> GSRPSTAKPSKIPTPQRKSPASKLDKSS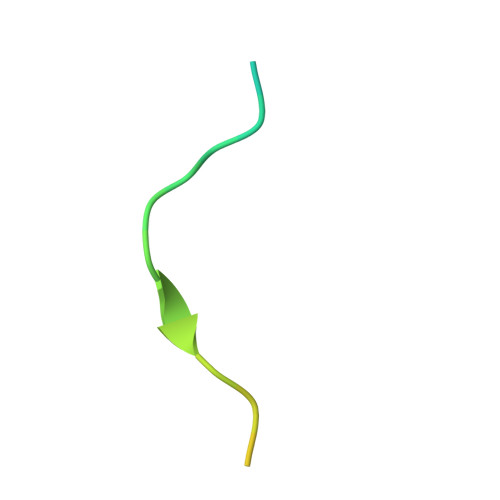KR1-adamantyl-[4-(5-chloranyl-2-methyl-phenyl)piperazin-1-yl]methanone 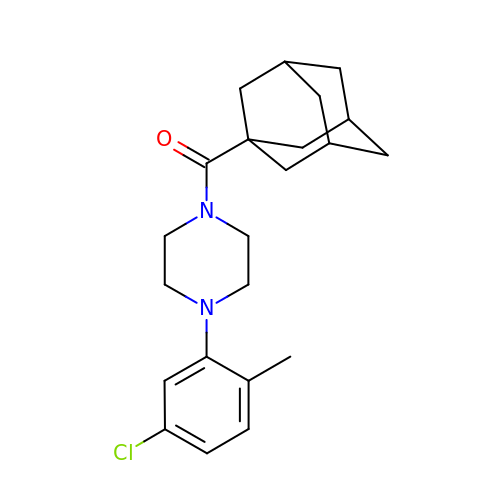| C22 H29 Cl N2 O | ZIJGUWNTLOYDSF-MAMSFEPMSA-N> PISPIETVPVKLKPGMDGPKVKQWPLTEEKIKALVEICTEMEKEGKISKIGPENPYNTPVFAIKKKDSTKWRKLVDFRELNKRTQDFWEVQLGIPHPAGLKKKKSVTVLDVGDAYFSVPLDEDFRKYTAFTIPSINNETPGIRYQYNVLPQGWKGSPAIFQSSMTKILEPFKKQNPDIVIYQYMDDLYVGSDLEIGQHRTKIEELRQHLLRWGLTTPDKKHQKEPPFLWMGYELHPDKWTVQPIVLPEKDSWTVNDIQKLVGKLNWASQIYPGIKVRQLCKLLRGTKALTEVIPLTEEAELELAENREILKEPVHGVYYDPSKDLIAEIQKQGQGQWTYQIYQEPFKNLKTGKYARMRGAHTNDVKQLTEAVQKITTESIVIWGKTPKFKLPIQKETWETWWTEYWQATWIPEWEFVNTPPLVKLWYQLEKEPIVGAETFYVDGAANRETKLGKAGYVTNKGRQKVVPLTNTTNQKTELQAIYLALQDSGLEVNIVTDSQYALGIIQAQPDKSESELVNQIIEQLIKKEKVYLAWVPAHKGIGGNEQVDKLVSAGIRKIL;> PISPIETVPVKLKPGMDGPKVKQWPLTEEKIKALVEICTEMEKEGKISKIGPENPYNTPVFAIKKKDSTKWRKLVDFRELNKRTQDFWEVQLGIPHPAGLKKKKSVTVLDVGDAYFSVPLDEDFRKYTAFTIPSINNETPGIRYQYNVLPQGWKGSPAIFQSSMTKILEPFKKQNPDIVIYQYMDDLYVGSDLEIGQHRTKIEELRQHLLRWGLTTPDKKHQKEPPFLWMGYELHPDKWTVQPIVLPEKDSWTVNDIQKLVGKLNWASQIYPGIKVRQLCKLLRGTKALTEVIPLTE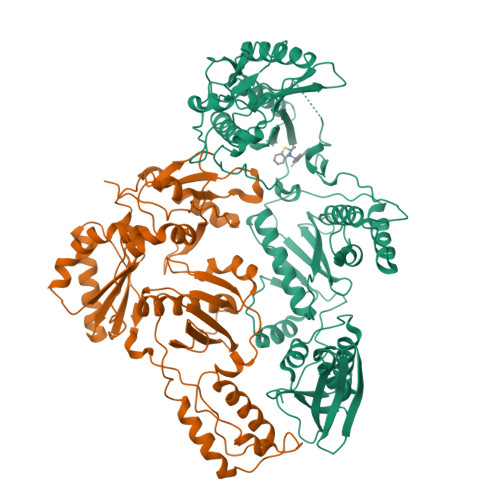EAELELAENREILKEPVHGVYYDPSKDLIAEIQKQGQGQWTYQIYQEPFKNLKTGKYARMRGAHTNDVKQLTEAVQKITTESIVIWGKTPKFKLPIQKETWETWWTEYWQATWIPEWEFVNTPPLVKLWYQLEKEPIVGAETF>ATALTNLVAEPFAKLEQDFGGSIGVYAMDTGSGATVSYRAEERFPLCGSFKGFLAAAVLARSQQQAGLLDTPIRYGKNALVPWSPISEKYLTTGMTVAELSAAA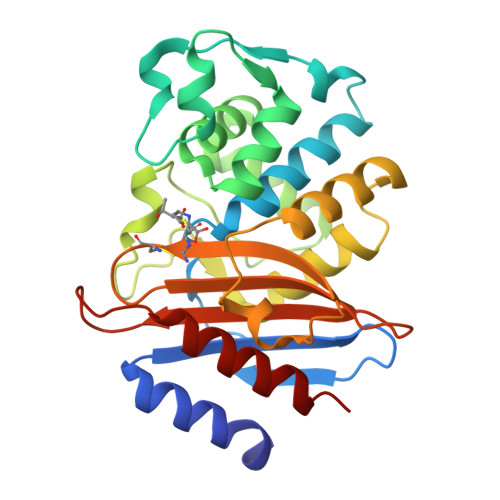VQYSDNAAANLLLKELGGPAGLTAFMRSIGDTTFRLDRWELELNSAIPGDARDTSSPRAVTESLQKLTLGSALAAPQRQQFVDWLKGNPTGNHRIRAAVPADWAVGDKTGTCGVYGTANDYAVVWPTGRAPIVLAVYTRAPNKDDKHSEAVIAAAARLALEGLG[2x]> MSLTKIPENV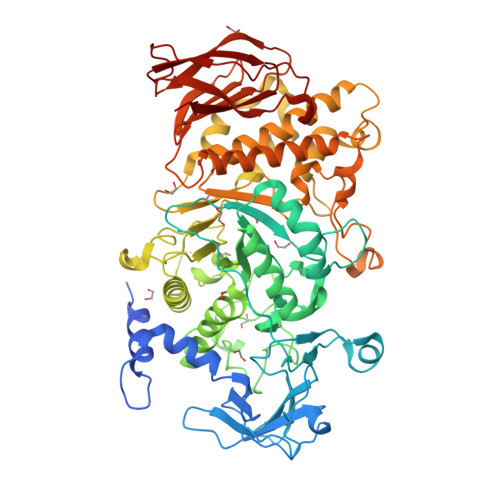QGAVSIDPWLEPFADVLSERRYLADKWLYDIKHATPDGSEQSLVDFARNAYKTYGLHANQQTKEIVYREWAPNAQRAFLVGEFNNWNEESHEMKHKDEFGVFSITLAPLENGDFAIPHDSKIKVMFVLPDGSKVYRIPAWITRATQPSKETAQKYGPTYEGRFWNPPNSYQFKHQRPKFNLANDSIKIYEAHIGISSPEPKVASYKEFTQNVLPRIKHLGYDAIQLMAIMEHAYYASFGYQVTNFFAISSRYGTPEDLKELIDTAHSMGILVLLDVIHSHASKNSEDGLNMFDGSDHQYFHSLTSGRGEHPLWDSRLFNYGSFEVQRFLLANLAYYIDVYQFDGFRFDGVTSMLYLHHGVGAGGAFSGDYNEYLSRDRSGVDHEALAYLMLANDLVHDLLPESAVTIAEDVSGYPTLCLPRTAGGGGFDYRLAMALPDMWIKLLKTKQDDDWDMGHIVHTLTNRRHGEKVVAYCESHDQALVGDKTLAFWLMDAAMYTDMTVLKEPTLVIDRGIALHKMIRLITHSLGGEAYLNFEGNEFGHPEWLDFPRVGNNDSYHYARRQFNLVDDDLLRYRHLNEFDAAMQNCESKHQWLNTPQAYVSLKHEVDKVIAFERNGHLFVFNFHPTQSFTDYRIGVDVAGTYKIVLNTDRAEFGGHNRIDEAQEFFTTDLEWNNRRNFIQVYIPSRTAIVLTRQM>[6x]QRSTPAITLESPDIKYPLRLIDREIISHDTRRFRFALPSPQHILGLPVGQHIYLSARIDGNLVVRPYTPISSDDDKGFVDLVIKVYFKDDHPKFPAGGKMSQYLESMQIGDTIEFRGPSGLLVYQGKGKFAIRPDKKSNPIIRTVKSVGMIAGG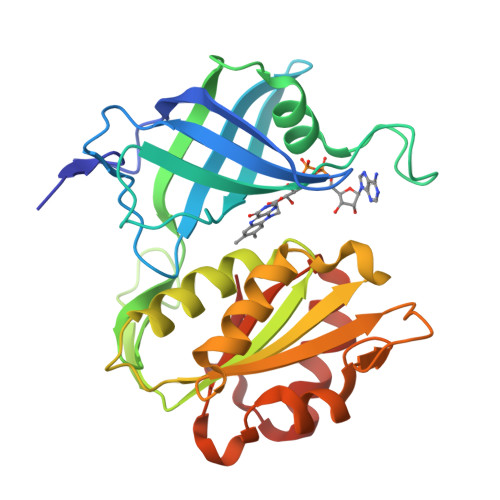TGITPMLQVIRAIMKDPDDHTVCHLLFANQTEKDILLRPELEELRNKHSARFKLWYTLDRAPEAWDYGQGFVNEEMIRDHLPPPEEEPLVLMCGPPPMIQYACLPNLDHVGHPTERCFVF Steroidogenic acute regulatory (StAR) protein related lipid transfer (START) domains are small globular modules that form a cavity where lipids and lipid hormones bind. The ∼210 residue globular START module is a curved β-sheet gripped by two α-helices. The concave face of the β-sheet and the C-terminal α-helix enclose a hydrophobic cavity that can accommodate lipid molecules. Here we present crystal structures of four human START domains, those of STARD1, STARD5, STARD13 and STARD14/ACOT11.

Group 2 consist of proteins containing only a START domain; group 3 proteins are capable of binding different ligands, such as phosphatidyl choline (STARD2/PCTP) and ceramides (STARD11); group 4 proteins (DLC, or deleted in cancerous liver cells) are frequently de-regulated in cancer and contain Rho-GTPase activating domains; group 5 proteins contain two thioesterase domains; and group 6 consists of only STARD9, a 4614-residue protein with unknown function, that contains a kinesin motor domain at its N-terminus. Of particular interest in the scope of this paper are STARD13 and STARD14, the family members for which the ligands are not known. STARD13 Arg974/STARD14 Arg449144 is highly conserved and is likely a key residue binding negatively charged lipids such as phosphatidylcholine and fatty acids. Based on our structural analysis we propose charged lipids as ligands for STARD13 and fatty acids as ligands for STARD14. All structures reported are relevant to disease. They are down- (STARD13) or up-regulated (STARD5) in cancers, mutations in them result in metabolic disorders (STARD1) or they are linked to obesity (STARD14;).

>SMRPQPGDGERRYREASARKKIRLDRKYIVSCKQTEVPLSVPWDPSNQVYLSYNNVSSLKMLVAKDNWVLSSEISQVRLYTLEDDKFLSFHMEMVVHVDAAQAFLLLSDLRQRPEWDKHYRSVELVQQVDEDDAIYHVTSPALGGHTKPQDFVILASRRKPCDNGDPYVIALRSVTLPTHRETPEYRRGETLCSGFCLWREGDQLTKVSYYNQATPGVLNYVTTNVAGLSSEFYTTFKACEQFLLDNRNDLAPSLQTL[2x]>LPQMTQQLNSDDMQEQLSATVKFRQILSREHRPPIDVVIQAGV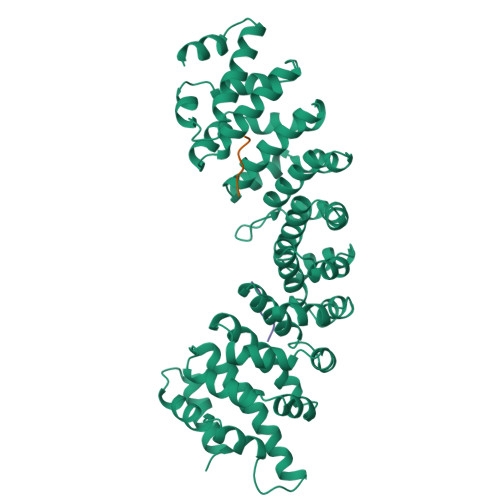VPRLVEFMRENQPEMLQLEAAWALTNIASGTSAQTKVVVDADAVPLFIQLLYTGSVEVKEQAIWALGNVAGDSTDYRDYVLQCNAMEPILGLFNSNKPSLIRTATWTLSNLCRGKKPQPDWSVVSQALPTLAKLIYSMDTETLVDACWAISYLSDGPQEAIQAVIDVRIPKRLVELLSHESTLVQTPALRAVGNIVTGNDLQTQVVINAGVLPALRLLLSSPKENIKKEACWTISNITAGNTEQIQAVIDANLIPPLVKLLEVAEYKTKKEACWAISNASSGGLQRPDIIRYLVSQGCIKPLCDLLEIADNRIIEVTLDALENIIKMGEADKEARGLNINENADFIEKAGGMEKIFNCQQNENDKIYEKAYKIIETYFG[2x];>KKKRKV[2x];>[2x]AKKAA> MPMASEESQAFQRQLTALIGYDVTDVSNVHDDELEFTRRGLVTPRMAEVASRDPKLYAMHPWVTSKPLPEYLWKKIANNCIFIVIHRSTTSQTIKVSPDDTPGAILQSFFTKMAKKKSLMDIPESQSEQ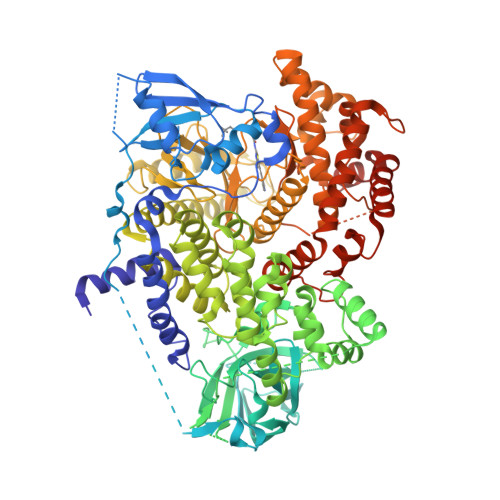DFVLRVCGRDEYLVGETPIKNFQWVRHCLKNGEEIHVVLDTPPDPALDEVRKEEWPLVDDCTGVTGYHEQLTIHGKDHESVFTVSLWDCDRKFRVKIRGIDIPVLPRNTDLTVFVEANIQHGQQVLCQRRTSPKPFTEEVLWNVWLEFSIKIKDLPKGALLNLQIYCGKAPALSSKASAESPSSESKGKVQLLYYVNLLLIDHRFLLRRGEYVLHMWQISGKGEDQGSFNADKLTSATNPDKENSMSISILLDNYCHPIALPKHQPTPDPEGDRVRAEMPNQLRKQLEAIIATDPLNPLTAEDKELLWHFRYESLKHPKAYPKLFSSVKWGQQEIVAKTYQLLARREVWDQSALDVGLTMQLLDCNFSDENVRAIAVQKLESLEDDDVLHYLLQLVQAVKFEPYHDSALARFLLKRGLRNKRIGHFLFWFLRSEIAQSRHYQQRFAVILEAYLRGCGTAMLHDFTQQVQVIEMLQKVTLDIKSLSAEKYDVSSQVISQLKQKLENLQNSQLPESFRVPYDPGLKAGALAIEKCKVMASKKKPLWLEFKCADPTALSNETIGIIFKHGDDLRQDMLILQILRIMESIWETESLDLCLLPYGCISTGDKIGMIEIVKDATTIAKIQQSTVGNTGAFKDEVLNHWLKEKSPTEEKFQAAVERFVYSCAGYCVATFVLGIGDRHNDNIMITETGNLFHIDFGHILGNYKSFLGINKERVPFVLTPDFLFVMGTSGKKTSPHFQKFQDICVKAYLALRHHTNLLIILFSMMLMTGMPQLTSKEDIEYIRDALTVGKNEEDAKKYFLDQIEVCRDKGWTVQFNWFLHLVLGIKQGEKHSALEHHHHHH We recently reported that the mitochondrial 2-Cys Prx of Leishmania infantum (mTXNPx, Prx1m) also adopts two functions, as a peroxidase and as a molecular chaperone. The catalytic activity of 2-Cys-peroxiredoxins (from hereon abbreviated as Prx), which comprise the Prx1 family, is mediated by the active site peroxidatic cysteine Cp, which reacts with peroxide and related oxidants, and undergoes reversible sulfenic acid formation. Once activated by elevated temperatures, reduced mTXNPx decamers protect a range of proteins from heat-induced aggregation both in vitro and in vivo. To obtain insights into the structural basis and mechanism of mTXNPx chaperone activity, we have now determined the cryo-EM structures of reduced, heat-activated mTXNPx with and without a bound model client protein to 3.7 and 2.9 Å resolution, respectively.

We determined 3D reconstructions of mTXNPxred incubated with and without luciferase, which yielded structures at 3.7 and 2.9 Å estimated resolution, respectively. 2D class averages revealed well-defined features of the decamer ring and a globular, central density that was present only after incubation with thermally unfolded luciferase. The overall size of the central density attributed to luciferase was consistent with a single 63 kDa luciferase molecule. Local resolution analysis identified uniform higher resolution (~3.6 Å) for the core of the mTXNPx ring and lower resolution regions for the inner face of the ring (i.e., 4.4 Å), indicating structural flexibility in proximity to the bound client. Remarkably, in the cryo-EM structure of client-bound mTXNPxred, we identified an additional inner ring of density that extends from position T35 and encapsulates the client density. Residues Q31-T35 of mTXNP were modeled into this density and identified to extend from each peroxiredoxin monomer at the dimer interface to form the inner ring. Based on the position of the N-terminal extensions, residues Y33 and R34 appear to contact the bound client along with additional residues in the N-terminal strand of the chaperone that were unable to be modeled. When refinements were performed without imposing symmetry (C1), the density projections remained present, indicating that all subunits likely make bona fide contact with the client, although some variability is observed. Thus, we conclude that the luciferase client is likely bound heterogeneously and in an unstructured state that, as previously shown, is competent for re-folding. We found that the N-terminal extensions of mTXNPxred become ordered upon client binding, and directly contact and encapsulate the client.

>MLRRLPTSCFLKRSQFRGFAATSPLLNLDYQMYRTATVREAAPQFSGQAVVNGAIKDINMNDYKGKYIVLFFYPMDFTFVCPTEIIAFSDRHADFEKLNTQVVAVSCDSVYSHLAWVNTPRKKGGLGEMHIPVLADKSMEIARDYGVLIEESGIALRGLFIIDKKGILRHSTINDLPVGRNVDEALRVLEAFQYADENGDAIPCGWKPGQPTLDTTKAGEFFEKNM[10x]The genes encoding dihydrouridine synthases (Dus) have been identified in yeast Saccharomyces cerevisiae and Escherichia coli. These enzymes are homologous to dihydroorotate dehydrogenases and dihydropyrimidine dehydrogenases and they use a flavin mononucleotide (FMN) to catalyze hydride transfer from NAD(P)H to the uridine substrate. The human enzyme conserves the ‘bona fide’ Dus domain that spans the first 330 amino acids, while a presumably unstructured linker (residues 331–367) connects the latter to an unprecedented double-stranded RNA binding domain (dsRBD) formed by residues 368 to 433. Using biochemical analysis and structural characterization, we here show that HsDus2 uses a unique strategy for binding and modifying its tRNA substrate. In contrast to other Dus proteins, HsDus2 has a dsRBD, which is the primary tRNA binding site.

Overall, the dsRBD structure contains an N-terminal extension (from Ser350 to residue 368) and the canonical αβββα topology (from Thr369 to Gly435). The N-terminal extension wraps the entire dsRBD, thus leading to a globular shape of the domain. This extension is made of a short β strand (β1) that interacts with the βββ fold, thereby forming an extended β-sheet followed by a long unstructured linker and a short α−helical turn (η1). The helices of the αβββα canonical fold pack against three antiparallel β strands as generally observed in classical dsRBDs such as in Xrpa. However, some variations are observed, notably a shorter β3 sheet and β1−β2 loop. Lys371, Lys419 and Lys420, located in conserved motifs as well as Arg397 are conserved basic residues among the dsRBDs and they are known to participate in the interaction with the dsRNA. To illustrate how the dsRBD of HsDus2 might bind its tRNA substrate which contains some dsRNA regions, a structural alignment of HsDus2dsRBD with the dsRBD of Xenopus leavis RNA binding protein A in complex with dsRNA was achieved. In the resulting model the dsRNA interacts with the protein via a ∼14 nucleotides-fragment, which can also be seen as the double-stranded region of the tRNA substrate corresponding to the acceptor and T-psi arm. The model also shows that the N-terminal extension does not interact with RNA suggesting its availability for protein-protein interaction. Remarkably, HsDus2dsRBD was also able to bind tRNA with an affinity in the same range of that of wild-type HsDus2 being ∼5–6 μM.

>MTSEQTGEPAEDTSGVIKMAVKFDRRAYPAQITPKMCLLEWCRREKLAQPVYETVQRPLDRLFSSIVTVAEQKYQSTLWDKSKKLAEQAAAIVCLRSQGLPEGRLGEESPSLHKHHHHHH[3x]N-hydroxy-1-{[4-(hydroxycarbamoyl)phenyl]methyl}-1H-indole-6-carboxamide 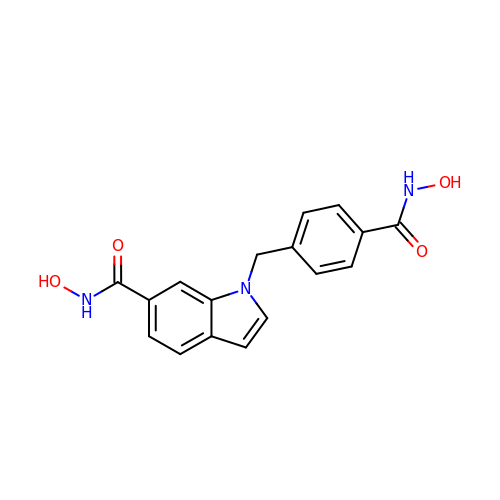| C17 H15 N3 O4 | IRJZGNPPEWBPKI-UHFFFAOYSA-N> SQIPASEQETLVRPKPLLLKLLKSVGAQKDTYTMKEVLFYLGQYIMTKRLYDEKQQHIVYCSNDLLGDLFGVPSFSVKEHRKIYTMIYRNLVVVNQQESSDSGTSV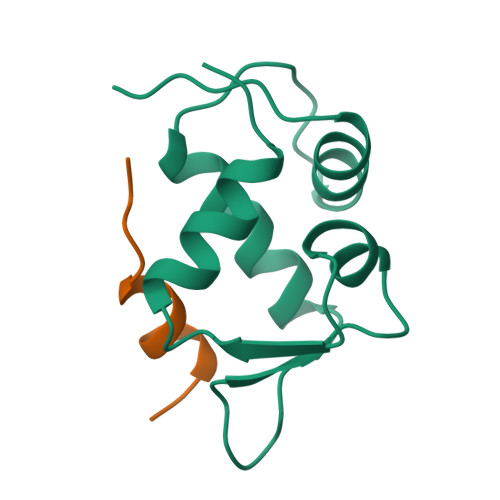SEN;> SQETFSDLWKLLPEN>[8x]TGGVQTVTLIPGDGIGPEISAAVMKIFDAAKAPIQWEERNVTAIQGPGGKWMIPSEAKESMDKNKMGLKGPLKTPIAAGHPSMNLLLRKTFDLYANVRPCVSIEGYKTPYTDVNIVTIRENTEGEYSGIEHVIVDGVVASIKLITEGASKRIAEFAFEYARNNHRSNVTAVHKANIMRMSDGLFLQKCREVAESCKDIKFNEMYLDTVCLNMVQDPSQFDVLVMPNLYGDILSDLCAGLIGGLGVTPSGNIGANGVAIFESVHGTAPDIAGKDMANPTALLLSAVMMLRHMGLFDHAARIEAACFATIKDGKSLTKDLGGNAKCSDFTEEICRRVKDLD;>ASRSQAEDVRVEGSFPVTMLPGDGVGPELMHAVKEVFKAAAVPVEFQEHHLSEVQNMASEEKLEQVLSSMKENKVAIIGKIHTPMEYKGELASYDMR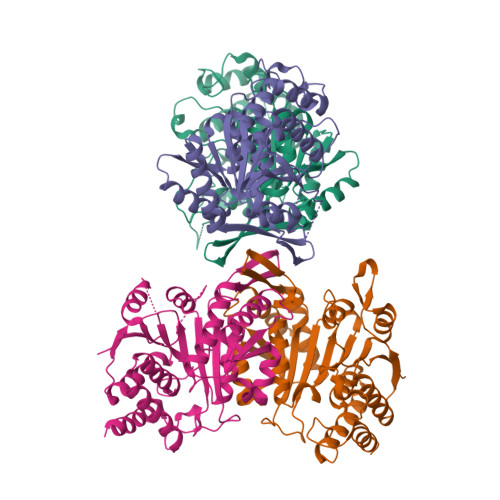LRRKLDLFANVVHVKSLPGYMTRHNNLDLVIIREQTEGEYSSLEHESARGVIECLKIVTRAKSQRIAKFAFDYATKKGRGKVTAVHKANIMKLGDGLFLQCCEEVAELYPKIKFETMIIDNCCMQLVQNPYQFDVLVMPNLYGNIIDNLAAGLVGGAGVVPGESYSAEYAVFETGARHPFAQAVGRNIANPTAMLLSASNMLRHLNLEYHSSMIADAVKKVIKVGKVRTSDMGGYATCHDFTEEICRRVKDLDEN[8x]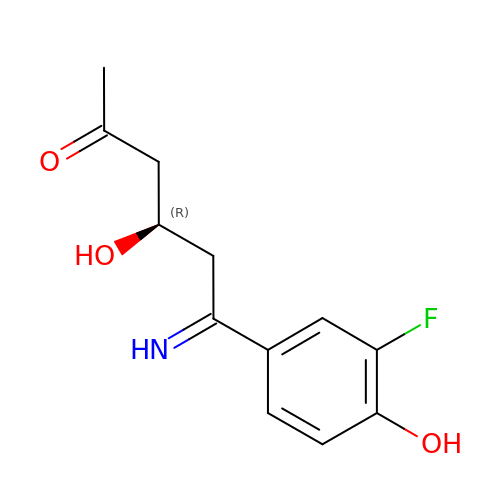(4R,6Z)-6-(3-fluoro-4-hydroxyphenyl)-4-hydroxy-6-iminohexan-2-one | C12 H14 F N O3 | DBWKEXPZAPNKOY-ZQQXWWNKSA-N> RAVTESAPNVEYHDVKGDMIQSVTTSFDDTSRLLTWTINLTPRQVKSNLGALV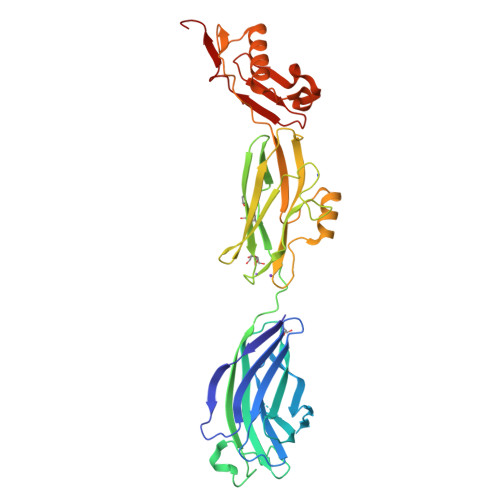SISGNQETRTVTINGKNAANGGVYNSGGAWNLYTGESVNNNVLRITTQVNDTGGEVKLGLRLVTSDKKITKTNLPLEFSQVAATTNGSWDKAGYNTTIVEKDTERPVVNVPSEITVYRGESFEYFATVTDNSNAFDLAKTVVRWLYSNQPGRGTEWLQYSVTQVGNQLKVRIFGNVPIDTTIGDYTRYVVATDAAGNVNATQTEMGNAAVDKTSVNGQFKLIIRFRIKTPENTVFVNNPNQLTEVEKNLVREAVKKSNPDLRAQDVLNSNYVTGITVSNNGTTTITYRDGRKDIIDGSKFIDTRAGS>GSHMDGLLNPRESSKFIAENSRDVFIDSGGVRRVAELLLAKAAGPELRVEGWKALHELNPRAADEAAVNWVFVTDTLNFSFWSEQDEHKCVVRYRGKTYSGYWSLCAAVNRALDEGIPITSASYYATVTLDQVRNILR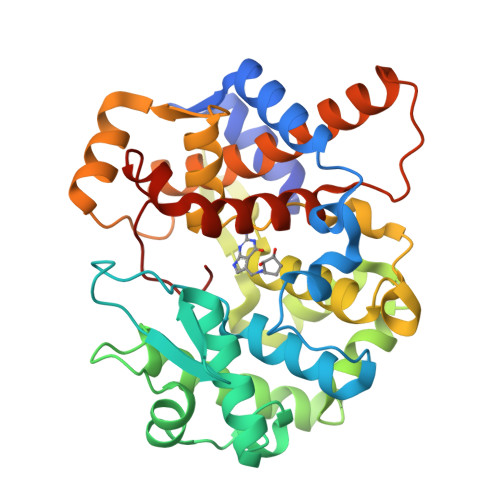SDTDVSMPLVEERHRILNETGKILLEKFGGSFLNCVRESENSAQKLMHLVVESFPSYRDVTLFEGKRVSFYKRAQILVADTWSVLEGKGDGCFKDISSITMFADYRLPQVLAHLGALKYSDDLLKKLLKGEMLSYGDRQEVEIRGCSLWCVELIRDCLLELIEQKGEKPNGEINSILLDYYLWDYAHDHREDMKGIPFHRIRCIYY[2x]(2S,5R)-1-formyl-5-[(sulfooxy)amino]piperidine-2-carbonitrile 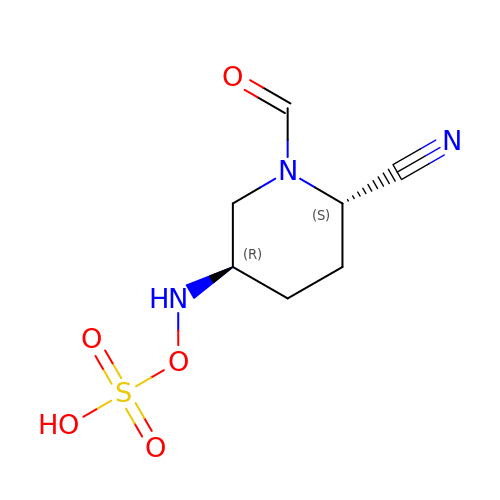| C7 H11 N3 O5 S | QMRJJHLCVKRXGQ-RQJHMYQMSA-N> GPHMGGSPGSVAENNLCSQYEEKVRPCIDLIDSLRALGVEQDLALPAIAVIGDQSSGKSSVLEALSGVALPRGSGIVTRCPLVLKLKKLVNEDKWRGKVSYQDYEIEISDASEVEKEINKAQNAIAGEGMGISHELITLEISSRDVPDLTLIDL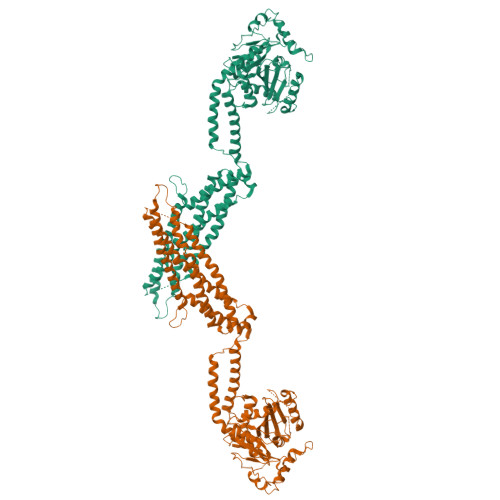PGITRVAVGNQPADIGYKIKTLIKKYIQRQETISLVVVPSNVDIATTEALSMAQEVDPEGDRTIGILTKPDLVDKGTEDKVVDVVRNLVFHLKKGYMIVKCRGQQEIQDQLSLSEALQREKIFFENHPYFRDLLEEGKATVPCLAEKLTSELITHICKSLPLLENQIKETHQRITEELQKYGVDIPEDENEKMFFLIDKVNAFNQDITALMQGEETVGEEDIRLFTRLRHEFHKWSTIIENNFQEGHKILSRKIQKFENQAAAAELPGFVNYRTFETIVKQQIKALEEPAVDMLHTVTDMVRLAFTDVSIKNFEEFFNLHRTAKSKIEDIRAEQEREGEKLIRLHFQMEQIVYGAFQSSSATDSSMEEIFQHLMAYHQEASKRISSHIPLIIQFFMLQTYGQQLQKAMLQLLQDKDTYSWLLKERSDTSDKRKFLKERLARLTQARRRLAQFPG> DYKDDDDKLVPRGSCHPRLSLHRPALEDLLLGSEANLTCTLTGLRDASGATFTWTPSSGKSAVQGPPERDLCGCYSVSSVLPGCAQPWNHGETFTCTAAHPELKTPLTANITKSGNTFRPEVHLLPPPSEELALNELVTLTCLARGFSPKDVLVRWLQGSQELPREKYLTWASRQEPSQGTTTYAVTSILRVAAEDWKKGE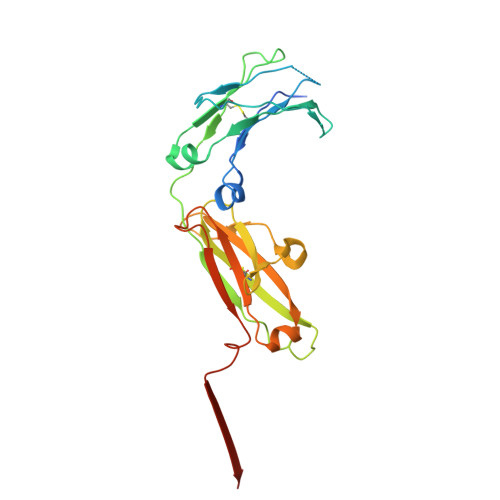TFSCMVGHEALPLAFTQKTIDRLAGKPTHINVSVVMAEADGTCY>MAHHHHHHMRITVDRSQFFKSLGRVHRVVERR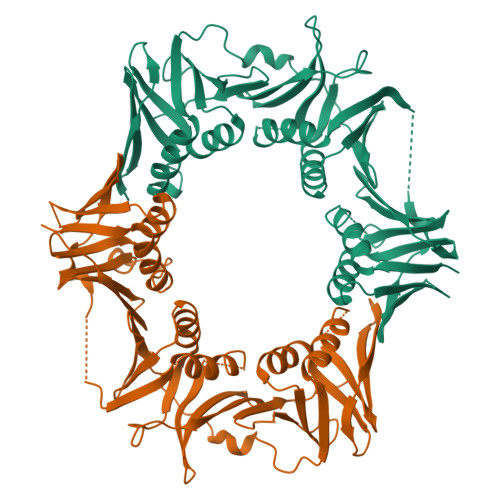NTVPILSNVLIDAENGSVQLKATDLDLEVTESFTVNIEKAGAITVPAYLLYDIVRKLPDGSEIVLSVDENQASAMSIVSGCTHFQLQCLPKIDFPESLPGQFGCRFFLSASKLKHLLDCTQFAISTEETRYYLNGIYFHIVHDDVLKLRLVATDGHRLAQVDMEAPSGVDGMPGVIIPRKAVGELQKLLSEEIDGDVCIELSETKIRFSLGSVVFTSKLVDGTFPDYQRVIPLGNDRKLIVNRQDFSSAVDRVSTISNDRGRAVKLTIEHGQLKLVVNNPDSGSAEDQLAATYTSEPLEIGFNSRYLLDIAGQLSSDEMVFMLSDAVAPALIRDNNNAEVLYVLMPVRV[2x]>MARKYFVAANWKCNGTLESIKSLTNSFNNLDFDPSKLDVVVFPVSVHYDHTRKLLQSKFSTGIENVSKFGNGSYTGEVSAEIAKDLNIEYVIIGHFERRKYFHETDEDVREKLQASLKNNLKAVVCFGESLEQREQNKTIEVITKQVKAFVDLIDNFDNVILVYEPLWAIGTGKTATPEQAQLVHKEIRKIVKDTCGEKQANQIRILYGGSVNTENCSSLIQQEDIDGFLVGNASLKESFVDII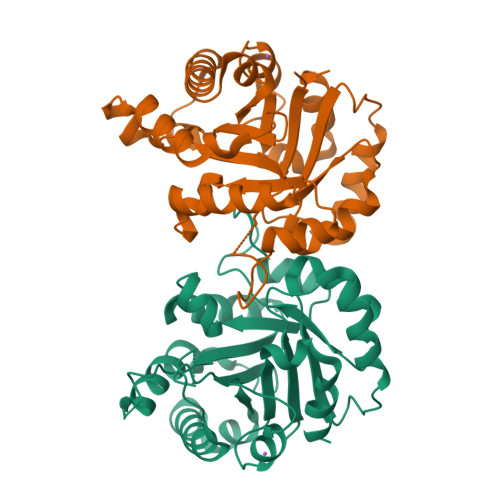KSAM[2x]> GPLGSAYMSRRESINPWILTGFADAEGSFLLRIRNNNKSSVGYSTELGFQITLHNKDKSILENIQSTWKVGVIANSGDNAVSLKVTRFEDLKVIIDHFEKYPLITQKLGDYMLFKQAFCVMENKEHLKINGIKELVRIKAKLNWGLTDELKFAFPEIISKERSLINKNIPNFKWLAGFTSGEGCFFVNLIKSKSKLGVQVQLVFSITQHIKDKNLMNSLITYLGCGYIKEKNKSEFSWLDFVVTKFSDINDKIIPVFQENTLIGVKLEDFEDWCKVAKLIEEK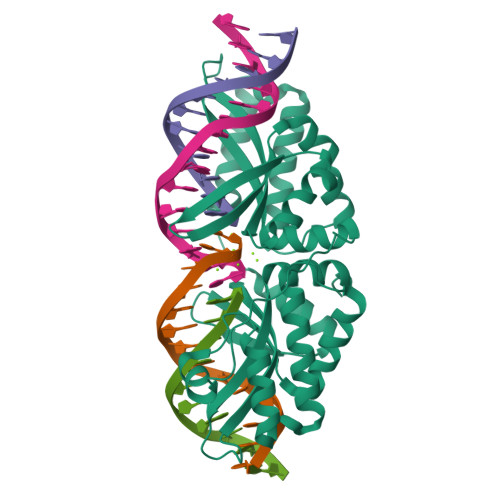KHLTESGLDEIKKIKLNMNKGRVF Parallel to this two other proteins have emerged – primarily from genetic studies – as being factors that significantly modulate plasma triglyceride levels and CAD. These proteins, human angiopoietin-like protein 3 (Angptl3; also known as Ang5) and angiopoietin-like protein 4 (Angptl4) are, as the names suggest, related structurally to angiopoietins which are involved in angiogenesis via their interaction with the Tie2 (tyrosine kinase with immunoglobulin and endothelial growth factor homology domain-2) receptor. Here we determined the structures of the fibrinogen-like domains of Angptl3 and Angptl4, structures which offer new insights into reported loss of function mutations, the mechanisms of action of the proteins and open up the possibility of rational design of low molecular weight inhibitors. The fibrinogen-like domains of Angptl3 and Angptl4 form compact structures and, according to fibrinogen nomenclature, can be divided to 3 subdomains A, B and P.

There are 3 monomers of Angptl3 in the asymmetric unit. In addition, there are two regions within the fibrinogen-like domain (Lys389 - His391 and Pro420 - Arg429 in the A-chain) for which the electron density is either missing or not of sufficient quality to allow tracing of the chain, suggesting the presence of flexible loops. In Angptl3, it is composed of five β-strands (β3, β4, β5, β6 and β10) forming a large twisted antiparallel β-sheet, and three α-helices (α2, α3 and α4). In Angptl3, the P subdomain contains little regular secondary structure - three short β-strands (β7, β8 and β9) and a short α-helix (α5). β7 and β8 form a small antiparallel β-hairpin, which is braced together with α5 and stabilized by a disulfide bond between Cys394 and Cys408. Angptl3 can be superimposed on its closest structural homologues, identified by Dali server, Angiopoietins 1 and 2 with a rms deviation of 2.3 Å (192 equivalent Cα positions; 4JYO40) or 2.4 Å (192 equivalent Cα positions; 1Z3S41) respectively. For example, the P subdomain of Angptl3 contains only 1 α-helical segment and 3 β-strands and does not superimpose well with structural homologs. In contrast, no distinct electrostatic properties were identified on the surface of the P subdomain of Angptl3. For Angptl3 there are twelve reported point mutations in the fibrinogen-like domain which are associated with decreased triglyceride levels - M259T, R288Q, S292P, E375K and Y417C, Y344S and, in decreasing order of severity, G253C, I333S, D290H, C408R, Y250C and T383S (;29 S292P also reported). Potential structural defects associated with seven of the other eight mutations can similarly be elucidated using the solved crystal structure, either from potential effects on intra- or inter-molecular disulfide bond formation (G253C, Y250C, C408R) and/or disruption of structure stabilizing sidechain or backbone hydrogen bonds (Y250C, D290H, I333S, T383S) and/or disruption of regular secondary structural elements (I333S, Y344S, T383S).

>MHHHHHHMIPAECTTIYNRGEHTSGMYAIRPSNSQVFHVYCDVISGSPWTLIQHRIDGSQNFNETWENYKYGFGRLDGEFWLGLEKIYSIVKQSNYVLRIELEDWKDNKHYIEYSFYLGNHETNYTLHLVAITGNVPNAIPENKDLVFSTWDHKAKGHFNCPEGYSGGWWWHDECGENNLNGKYNKPRAKSKPERRRGLSWKSQNGRLYSIKSTKMLIHPTDSESFE[3x]1,2,3,4-tetrahydroisoquinolin-8-amine 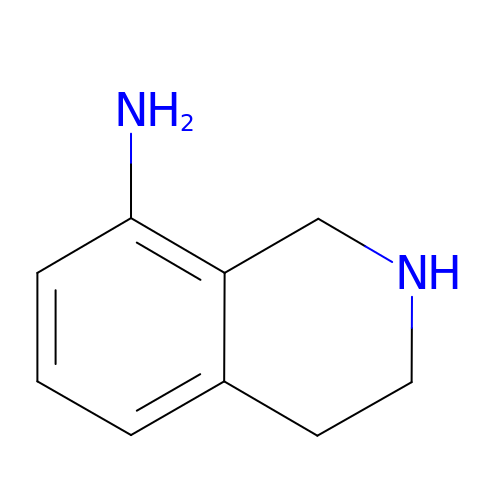| C9 H12 N2 | GIIQUGGTGRRQEN-UHFFFAOYSA-N> SNKVGTLQAQVEATQKQKAQPIDANRKYDYKLQYYLNDYVYAYFTLPQEGDKQQAQVEHLNSFYNFVPDVKAQGQVRNPSTLLDSQLVTVEGKVATYK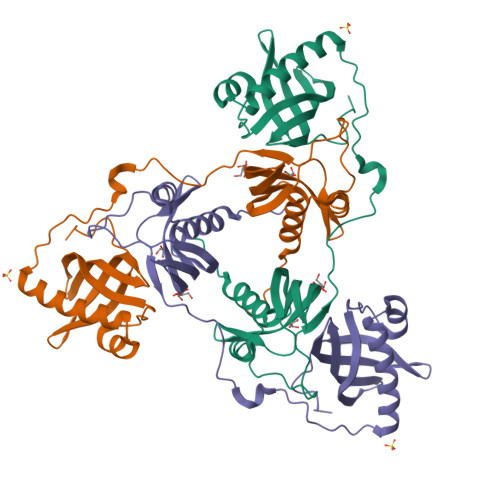VKYKEMIQHDKDTEEKELVTGFNIPFDEKEGKYYVSGLPWFSAIESSQAGYFSEDDQLQLTANDHVSDSQHKKVEKFLKVFFTNYTTNQDNLNLIAKNVAIVANTTFKTIDYTYLKKDRADLIAYVQATFEVGGTTHSENFTFTLSEKDKSYYVTKLEHTIPLNYANDKD> LS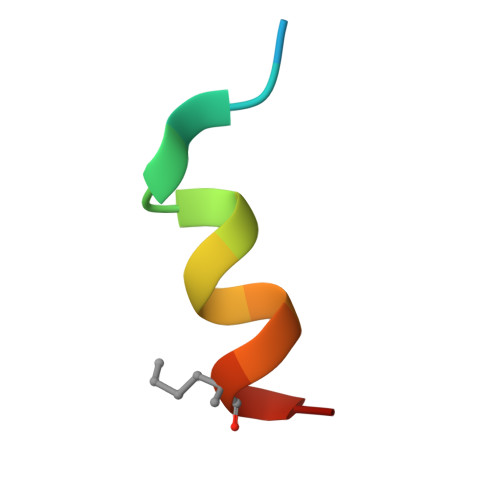QETFXDLWKLELENX>HHHHHHMSTKKKPTITKQELYSLVAADTQLNKALIERIFTSQQKIIQNALKHNQEVIIPPGIKFT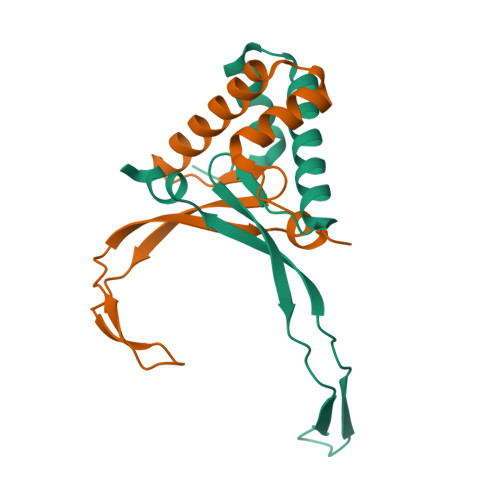VVTVKAKPARQGHNPATGEPIQIKAKPEHKAVKIRALKPVHDMLN[2x]> CATTAGCGTCAGACGATAAATTTAGCCGGAACTAAAACACTCTTGTATCATCGCCTTGTAGCG;> ATTAAAGATCGGCACGGAGATATCTTTGACCCCCACTAAAACCGCTTTT;> AAGGGCGACATTCAATAAGTTTACCAGAATGAAATTTTACAG;> TTTTTTTTTTTGGTTTACCAGCGCCACAATAGAAAGCAGA;> TTTTTTTTTTTAGTCAGAAGCAACTCCAACAGGTTTTTTTTTTT;> AAGCGGAGGAGAAGGAACCCTAAATCACCATCAATATGATTTTTTTTTTT;> TTGCATCAAATCAGTAAATATTCATTGACCAGAGGGGGTAATAGTAAAA;> CAAACGTGACTCCTCGCTAATTGAACAAAGTCAGACTCCTCA;> TATTTTGTCACAATAAGACAAGGAACCAGAGCCACCACCGTTTTTTTTTT;> AATTCGAGCTTCAAAGCGAACTCCTTTTCTGTAGCTCAACATGTTTTAA;> TGATAGACGGTTTTTCGCCCTTTGACGTTGGAGTCCACGTTCTTTAATAGTGGACTCTTGTTCCAAACTGGAACAACACTCAACCCTATCTCGGGCTATTCTTTTGATTTATAAGGGATTTTGCCGATTTCGGAACCACCATCAAACAGGATTTTCGCCTGCTGGGGCAAACCAGCGTGGACCGCTTGCTGCAACTCTCTCAGGGCCAG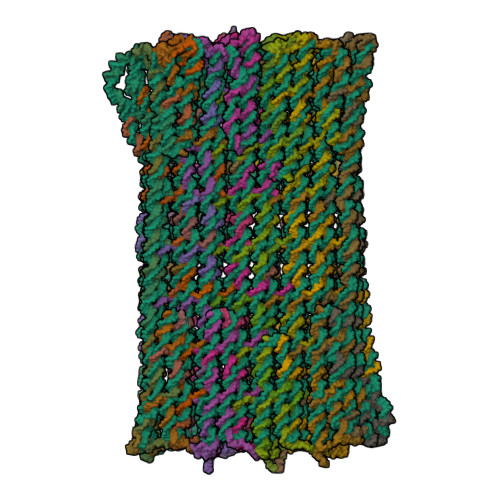GCGGTGAAGGGCAATCAGCTGTTGCCCGTCTCACTGGTGAAAAGAAAAACCACCCTGGCGCCCAATACGCAAACCGCCTCTCCCCGCGCGTTGGCCGATTCATTAATGCAGCTGGCACGACAGGTTTCCCGACTGGAAAGCGGGCAGTGAGCGCAACGCAATTAATGTGAGTTAGCTCACTCATTAGGCACCCCAGGCTTTACACTTTATGCTTCCGGCTCGTATGTTGTGTGGAATTGTGAGCGGATAACAATTTCACACAGGAAACAGCTATGACCATGATTACGAATTCGAGCTCGGTACCCGGGGATCCTCAACTGTGAGGAGGCTCACGGACGCGAAGAACAGGCACGCGTGCTGGCAGAAACCCCCGGTATGACCGTGAAAACGGCCCGCCGCATTCTGGCCGCAGCACCACAGAGTGCACAGGCGCGCAGTGACACTGCGCTGGATCGTCTGATGCAGGGGGCACCGGCACCGCTGGCTGCAGGTAACCCGGCATCTGATGCCGTTAACGATTTGCTGAACACACCAGTGTAAGGGATGTTTATGACGAGCAAAGAAACCTTTACCCATTACCAGCCGCAGGGCAACAGTGACCCGGCTCATACCGCAACCGCGCCCGGCGGATTGAGTGCGAAAGCGCCTGCAATGACCCCGCTGATGCTGGACACCTCCAGCCGTAAGCTGGTTGCGTGGGATGGCACCACCGACGGTGCTGCCGTTGGCATTCTTGCGGTTGCTGCTGACCAGACCAGCACCACGCTGACGTTCTACAAGTCCGGCACGTTCCGTTATGAGGATGTGCTCTGGCCGGAGGCTGCCAGCGACGAGACGAAAAAACGGACCGCGTTTGCCGGAACGGCAATCAGCATCGTTTAACTTTACCCTTCATCACTAAAGGCCGCCTGTGCGGCTTTTTTTACGGGATTTTTTTATGTCGATGTACACAACCGCCCAACTGCTGGCGGCAAATGAGCAGAAATTTAAGTTTGATCCGCTGTTTCTGCGTCTCTTTTTCCGTGAGAGCTATCCCTTCACCACGGAGAAAGTCTATCTCTCACAAATTCCGGGACTGGTAAACATGGCGCTGTACGTTTCGCCGATTGTTTCCGGTGAGGTTATCCGTTCCCGTGGCGGCTCCACCTCTGAAAGCTTGGCACTGGCCGTCGTTTTACAACGTCGTGACTGGGAAAACCCTGGCGTTACCCAACTTAATCGCCTTGCAGCACATCCCCCTTTCGCCAGCTGGCGTAATAGCGAAGAGGCCCGCACCGATCGCCCTTCCCAACAGTTGCGCAGCCTGAATGGCGAATGGCGCTTTGCCTGGTTTCCGGCACCAGAAGCGGTGCCGGAAAGCTGGCTGGAGTGCGATCTTCCTGAGGCCGATACTGTCGTCGTCCCCTCAAACTGGCAGATGCACGGTTACGATGCGCCCATCTACACCAACGTGACCTATCCCATTACGGTCAATCCGCCGTTTGTTCCCACGGAGAATCCGACGGGTTGTTACTCGCTCACATTTAATGTTGATGAAAGCTGGCTACAGGAAGGCCAGACGCGAATTATTTTTGATGGCGTTCCTATTGGTTAAAAAATGAGCTGATTTAACAAAAATTTAATGCGAATTTTAACAAAATATTAACGTTTACAATTTAAATATTTGCTTATACAATCTTCCTGTTTTTGGGGCTTTTCTGATTATCAACCGGGGTACATATGATTGACATGCTAGTTTTACGATTACCGTTCATCGATTCTCTTGTTTGCTCCAGACTCTCAGGCAATGACCTGATAGCCTTTGTAGATCTCTCAAAAATAGCTACCCTCTCCGGCATTAATTTATCAGCTAGAACGGTTGAATATCATATTGATGGTGATTTGACTGTCTCCGGCCTTTCTCACCCTTTTGAATCTTTACCTACACATTACTCAGGCATTGCATTTAAAATATATGAGGGTTCTAAAAATTTTTATCCTTGCGTTGAAATAAAGGCTTCTCCCGCAAAAGTATTACAGGGTCATAATGTTTTTGGTACAACCGATTTAGCTTTATGCTCTGAGGCTTTATTGCTTAATTTTGCTAATTCTTTGCCTTGCCTGTATGATTTATTGGATGTTAATGCTACTACTATTAGTAGAATTGATGCCACCTTTTCAGCTCGCGCCCCAAATGAAAATATAGCTAAACAGGTTATTGACCATTTGCGAAATGTATCTAATGGTCAAACTAAATCTACTCGTTCGCAGAATTGGGAATCAACTGTTATATGGAATGAAACTTCCAGACACCGTACTTTAGTTGCATATTTAAAACATGTTGAGCTACAGCATTATATTCAGCAATTAAGCTCTAAGCCATCCGCAAAAATGACCTCTTATCAAAAGGAGCAATTAAAGGTACTCTCTAATCCTGACCTGTTGGAGTTTGCTTCCGGTCTGGTTCGCTTTGAAGCTCGAATTAAAACGCGATATTTGAAGTCTTTCGGGCTTCCTCTTAATCTTTTTGATGCAATCCGCTTTGCTTCTGACTATAATAGTCAGGGTAAAGACCTGATTTTTGATTTATGGTCATTCTCGTTTTCTGAACTGTTTAAAGCATTTGAGGGGGATTCAATGAATATTTATGACGATTCCGCAGTATTGGACGCTATCCAGTCTAAACATTTTACTATTACCCCCTCTGGCAAAACTTCTTTTGCAAAAGCCTCTCGCTATTTTGGTTTTTATCGTCGTCTGGTAAACGAGGGTTATGATAGTGTTGCTCTTACTATGCCTCGTAATTCCTTTTGGCGTTATGTATCTGCATTAGTTGAATGTGGTATTCCTAAATCTCAACTGATGAATCTTTCTACCTGTAATAATGTTGTTCCGTTAGTTCGTTTTATTAACGTAGATTTTTCTTCCCAACGTCCTGACTGGTATAATGAGCCAGTTCTTAAAATCGCATAAGGTAATTCACAATGATTAAAGTTGAAATTAAACCATCTCAAGCCCAATTTACTACTCGTTCTGGTGTTTCTCGTCAGGGCAAGCCTTATTCACTGAATGAGCAGCTTTGTTACGTTGATTTGGGTAATGAATATCCGGTTCTTGTCAAGATTACTCTTGATGAAGGTCAGCCAGCCTATGCGCCTGGTCTGTACACCGTTCATCTGTCCTCTTTCAAAGTTGGTCAGTTCGGTTCCCTTATGATTGACCGTCTGCGCCTCGTTCCGGCTAAGTAACATGGAGCAGGTCGCGGATTTCGACACAATTTATCAGGCGATGATACAAATCTCCGTTGTACTTTGTTTCGCGCTTGGTATAATCGCTGGGGGTCAAAGATGAGTGTTTTAGTGTATTCTTTTGCCTCTTTCGTTTTAGGTTGGTGCCTTCGTAGTGGCATTACGTATTTTACCCGTTTAATGGAAACTTCCTCATGAAAAAGTCTTTAGTCCTCAAAGCCTCTGTAGCCGTTGCTACCCTCGTTCCGATGCTGTCTTTCGCTGCTGAGGGTGACGATCCCGCAAAAGCGGCCTTTAACTCCCTGCAAGCCTCAGCGACCGAATATATCGGTTATGCGTGGGCGATGGTTGTTGTCATTGTCGGCGCAACTATCGGTATCAAGCTGTTTAAGAAATTCACCTCGAAAGCAAGCTGATAAACCGATACAATTAAAGGCTCCTTTTGGAGCCTTTTTTTTGGAGATTTTCAACGTGAAAAAATTATTATTCGCAATTCCTTTAGTTGTTCCTTTCTATTCTCACTCCGCTGAAACTGTTGAAAGTTGTTTAGCAAAATCCCATACAGAAAATTCATTTACTAACGTCTGGAAAGACGACAAAACTTTAGATCGTTACGCTAACTATGAGGGCTGTCTGTGGAATGCTACAGGCGTTGTAGTTTGTACTGGTGACGAAACTCAGTGTTACGGTACATGGGTTCCTATTGGGCTTGCTATCCCTGAAAATGAGGGTGGTGGCTCTGAGGGTGGCGGTTCTGAGGGTGGCGGTTCTGAGGGTGGCGGTACTAAACCTCCTGAGTACGGTGATACACCTATTCCGGGCTATACTTATATCAACCCTCTCGACGGCACTTATCCGCCTGGTACTGAGCAAAACCCCGCTAATCCTAATCCTTCTCTTGAGGAGTCTCAGCCTCTTAATACTTTCATGTTTCAGAATAATAGGTTCCGAAATAGGCAGGGGGCATTAACTGTTTATACGGGCACTGTTACTCAAGGCACTGACCCCGTTAAAACTTATTACCAGTACACTCCTGTATCATCAAAAGCCATGTATGACGCTTACTGGAACGGTAAATTCAGAGACTGCGCTTTCCATTCTGGCTTTAATGAGGATTTATTTGTTTGTGAATATCAAGGCCAATCGTCTGACCTGCCTCAACCTCCTGTCAATGCTGGCGGCGGCTCTGGTGGTGGTTCTGGTGGCGGCTCTGAGGGTGGTGGCTCTGAGGGTGGCGGTTCTGAGGGTGGCGGCTCTGAGGGAGGCGGTTCCGGTGGTGGCTCTGGTTCCGGTGATTTTGATTATGAAAAGATGGCAAACGCTAATAAGGGGGCTATGACCGAAAATGCCGATGAAAACGCGCTACAGTCTGACGCTAAAGGCAAACTTGATTCTGTCGCTACTGATTACGGTGCTGCTATCGATGGTTTCATTGGTGACGTTTCCGGCCTTGCTAATGGTAATGGTGCTACTGGTGATTTTGCTGGCTCTAATTCCCAAATGGCTCAAGTCGGTGACGGTGATAATTCACCTTTAATGAATAATTTCCGTCAATATTTACCTTCCCTCCCTCAATCGGTTGAATGTCGCCCTTTTGTCTTTGGCGCTGGTAAACCATATGAATTTTCTATTGATTGTGACAAAATAAACTTATTCCGTGGTGTCTTTGCGTTTCTTTTATATGTTGCCACCTTTATGTATGTATTTTCTACGTTTGCTAACATACTGCGTAATAAGGAGTCTTAATCATGCCAGTTCTTTTGGGTATTCCGTTATTATTGCGTTTCCTCGGTTTCCTTCTGGTAACTTTGTTCGGCTATCTGCTTACTTTTCTTAAAAAGGGCTTCGGTAAGATAGCTATTGCTATTTCATTGTTTCTTGCTCTTATTATTGGGCTTAACTCAATTCTTGTGGGTTATCTCTCTGATATTAGCGCTCAATTACCCTCTGACTTTGTTCAGGGTGTTCAGTTAATTCTCCCGTCTAATGCGCTTCCCTGTTTTTATGTTATTCTCTCTGTAAAGGCTGCTATTTTCATTTTTGACGTTAAACAAAAAATCGTTTCTTATTTGGATTGGGATAAATAATATGGCTGTTTATTTTGTAACTGGCAAATTAGGCTCTGGAAAGACGCTCGTTAGCGTTGGTAAGATTCAGGATAAAATTGTAGCTGGGTGCAAAATAGCAACTAATCTTGATTTAAGGCTTCAAAACCTCCCGCAAGTCGGGAGGTTCGCTAAAACGCCTCGCGTTCTTAGAATACCGGATAAGCCTTCTATATCTGATTTGCTTGCTATTGGGCGCGGTAATGATTCCTACGATGAAAATAAAAACGGCTTGCTTGTTCTCGATGAGTGCGGTACTTGGTTTAATACCCGTTCTTGGAATGATAAGGAAAGACAGCCGATTATTGATTGGTTTCTACATGCTCGTAAATTAGGATGGGATATTATTTTTCTTGTTCAGGACTTATCTATTGTTGATAAACAGGCGCGTTCTGCATTAGCTGAACATGTTGTTTATTGTCGTCGTCTGGACAGAATTACTTTACCTTTTGTCGGTACTTTATATTCTCTTATTACTGGCTCGAAAATGCCTCTGCCTAAATTACATGTTGGCGTTGTTAAATATGGCGATTCTCAATTAAGCCCTACTGTTGAGCGTTGGCTTTATACTGGTAAGAATTTGTATAACGCATATGATACTAAACAGGCTTTTTCTAGTAATTATGATTCCGGTGTTTATTCTTATTTAACGCCTTATTTATCACACGGTCGGTATTTCAAACCATTAAATTTAGGTCAGAAGATGAAATTAACTAAAATATATTTGAAAAAGTTTTCTCGCGTTCTTTGTCTTGCGATTGGATTTGCATCAGCATTTACATATAGTTATATAACCCAACCTAAGCCGGAGGTTAAAAAGGTAGTCTCTCAGACCTATGATTTTGATAAATTCACTATTGACTCTTCTCAGCGTCTTAATCTAAGCTATCGCTATGTTTTCAAGGATTCTAAGGGAAAATTAATTAATAGCGACGATTTACAGAAGCAAGGTTATTCACTCACATATATTGATTTATGTACTGTTTCCATTAAAAAAGGTAATTCAAATGAAATTGTTAAATGTAATTAATTTTGTTTTCTTGATGTTTGTTTCATCATCTTCTTTTGCTCAGGTAATTGAAATGAATAATTCGCCTCTGCGCGATTTTGTAACTTGGTATTCAAAGCAATCAGGCGAATCCGTTATTGTTTCTCCCGATGTAAAAGGTACTGTTACTGTATATTCATCTGACGTTAAACCTGAAAATCTACGCAATTTCTTTATTTCTGTTTTACGTGCAAATAATTTTGATATGGTAGGTTCTAACCCTTCCATTATTCAGAAGTATAATCCAAACAATCAGGATTATATTGATGAATTGCCATCATCTGATAATCAGGAATATGATGATAATTCCGCTCCTTCTGGTGGTTTCTTTGTTCCGCAAAATGATAATGTTACTCAAACTTTTAAAATTAATAACGTTCGGGCAAAGGATTTAATACGAGTTGTCGAATTGTTTGTAAAGTCTAATACTTCTAAATCCTCAAATGTATTATCTATTGACGGCTCTAATCTATTAGTTGTTAGTGCTCCTAAAGATATTTTAGATAACCTTCCTCAATTCCTTTCAACTGTTGATTTGCCAACTGACCAGATATTGATTGAGGGTTTGATATTTGAGGTTCAGCAAGGTGATGCTTTAGATTTTTCATTTGCTGCTGGCTCTCAGCGTGGCACTGTTGCAGGCGGTGTTAATACTGACCGCCTCACCTCTGTTTTATCTTCTGCTGGTGGTTCGTTCGGTATTTTTAATGGCGATGTTTTAGGGCTATCAGTTCGCGCATTAAAGACTAATAGCCATTCAAAAATATTGTCTGTGCCACGTATTCTTACGCTTTCAGGTCAGAAGGGTTCTATCTCTGTTGGCCAGAATGTCCCTTTTATTACTGGTCGTGTGACTGGTGAATCTGCCAATGTAAATAATCCATTTCAGACGATTGAGCGTCAAAATGTAGGTATTTCCATGAGCGTTTTTCCTGTTGCAATGGCTGGCGGTAATATTGTTCTGGATATTACCAGCAAGGCCGATAGTTTGAGTTCTTCTACTCAGGCAAGTGATGTTATTACTAATCAAAGAAGTATTGCTACAACGGTTAATTTGCGTGATGGACAGACTCTTTTACTCGGTGGCCTCACTGATTATAAAAACACTTCTCAGGATTCTGGCGTACCGTTCCTGTCTAAAATCCCTTTAATCGGCCTCCTGTTTAGCTCCCGCTCTGATTCTAACGAGGAAAGCACGTTATACGTGCTCGTCAAAGCAACCATAGTACGCGCCCTGTAGCGGCGCATTAAGCGCGGCGGGTGTGGTGGTTACGCGCAGCGTGACCGCTACACTTGCCAGCGCCCTAGCGCCCGCTCCTTTCGCTTTCTTCCCTTCCTTTCTCGCCACGTTCGCCGGCTTTCCCCGTCAAGCTCTAAATCGGGGGCTCCCTTTAGGGTTCCGATTTAGTGCTTTACGGCACCTCGACCCCAAAAAACTTGATTTGGGTGATGGTTCACGTAGTGGGCCATCGCCC;> TTTTTTTTTTACTAAAGACTTTTTCATACAGAGGGAGCCT;> TTTTTTTTTTACAGACCAGGCGAGCTGCTCATTCTTTTTTTTTT;> CATAGGCTGGCTGATTTGAAAGAGGACAGATGAACGGTGTTTTTTTTTTT;> CCTTCATTTACCCAAACACCAAATTTCACCAGTCAGGACGTTGGGAA;> GGCTTGCGACAACATAAACAAGTCTTTCCAGACGTTAGTAAAGTATGGG;> CTCAGCAGAATTTCAACAACTCAGACAGCCCTCATAGTTAGCTGAGAAT;> AGGGTAGCAACGGCTGAGGAAGTTTCCATTAAACGCGGAACGTTATCAG;> GTTGCGCCGACAATAGGGAGTCAGAGCCCGTTTTCGTGAATTATCACAA;> ACCGATAAGCGGAGGTAACGATCTAAAGTTTTGTCCTTTCAA;> TTAAACAGCTTGATGCGGGATAGCCGCCTCATAGCGACGGAATTAGAGCCAGCA;> TTTTTTTTTTGCTCCAAAAGCTTTGAGGTTTTTTTTTT;> TTTTTTTTTTAGTGAATAAGGCGAATTACCTTATTTTTTTTTTT;> TAATAATTACAACGTTTCAGGGATAGCATACCGCC;> AATCTCCAGTTTCGTAGGAACCCATGTACCTTTTTTTTTT;> ACTTTAATCATTGTTTGCCCTAATTACGCGTTTACGAAGCAA;> TGAATGGGCTTGAGATGGTTTGAACGAGCAGATAC;> CCTGTAGCATTCCAAAAGGAAGGGTCAGAAAGCGCCGAGGAAAAAGACA;> TCACCAGTACAAACTTTTTCATACTGGTCCGTTCCACAAAGT;> TTTTTTTTTTGTAACACTGAAAAAAAAGTTTTTTTTTT;> AGCGCGAAACAAAGTACAATTTTCGGACCAGAAAAATAAATATAAAC;> ACCTGCTCCCAATCATACCGATATATTCGGCAGGAGG;> GAAAAATCTACGTTCAACTTATAATGGATAAGAAATAGTATAAAGCTAAATCGG;> TTTTTTTTTTCCGTACTCAGGAGGTTTAGAGCCCAA;> TTTTTTTTTTGCGATTTTAAGAACTGGCTTAACGGA;> ACCCTCAGAGCCACCACACCCTCTGCCGTCAACATAAAAGAGCA;> TTTTTTTTTTTAGAAAGATGTAAGAGCATTTTTTTTTT;> TTGAGATTTAGGAACAAAAGGGACGAGAAATCAACGTAACAA;> GGGTTTTGCTCAGTATTAGACAATTGAGTTTTATTCAAGAAATCATTTG;> GAGAGGGTTTAACGTTGCGAACTTGCTTTCGAGGTGCGAAAG;> AAGTATAAGCAGCCAGCAATATATTAAAACCAATCAAACAAA;> GCCCGGAAGGAGTGCGTTGAATTAATTGTATCGGT;> AGGCATATCATCAGACAACATTATTACAGGTTTTTTTTTT;> TCTGAAACATGATGTAGTAAAGAACCGGATATTCACAAGAGT;> CTATTATGGCAGGTCAATATCGCGTTTTTTTGCGGATGGCGT;> TCGGAACATTTTGCACCATCGCCCACGCATAACAATTTTTCT;> GCCCCCTTGATATTTGATTAAAGAAAATCAGACGAAGTATCA;> GTGCCCGTCCTCATGAATACCGGCAACAAAAAGGTATTCTTA;> TTTTTTTTTTTTTTGATGATACATAGGTGTATCATTTTTTTTTT;> TTTTTTTTTTACACTATCAACTGGATAGTTTTTTTTTT;> CAGACGACGATAAAATAACGCTACCACATTAATAAAACGAACCATTATA;> AACCAAAATAGCGACAAAAGAAATCTTGAAGGGAACCGAACTGACCAAC;> TAAAGCCCCCTCAGCGTCACCACGAAGGCACCAACGCGATTATACCA;> GAATTTAAATAAGTTTGATATACCCTCAGAACCGCCCCTCAT;> AGTTTTGATCCCCCTGACCATAAATCAAAAAAAGATTAAGAG;> GCATTGATCGCTGAGAGGCGCAGACGGTATGTTACTGTGTCGAAATCCGCG;> GCCGCCATTGGCCTGCCTATTAGAGAAGGATTAGGAACACCCATCAGAG;> GCCACCAAGAATGGTGCCTTGGGATAAGAGAACCGCC;> CCTCAGATTGCCATGAGGGAGGGAAGGTGAAACGCACGCAAT;> TTTTTTTTTTGAACCGCCTCCCGTCATACATGGCTTTTTTTTTT;> TTTTTTTTTTCGTCCAATACTGCGGATGTTTAGTAACCCT;> ATCGTCAGTCTTTACCCTGACTATTATTTTTTTTTT;> GATTAAGAATCATATCGCCATATTTAACAACGCTTTTTTTTTT;> AGGTCATTGCCTGAAGAGGGTAACCAGGCAGCTGGTGGGTAACGCCAGG;> TTTTTTTTTTTACCTGAGCGAAGAGTCATTTTTTTTTT;> TTTTTTTTTTTAATCGTAAAACATTTTGTTAAAATTTTTTTTTT;> TATGTACATTTAAACTCATTTTTTAACCGGCCTTC;> ACATCGGTTTTTTAAGATAAGTTCTGTCACATACA;> CTGATTGTTTGCACGTAAAACTCCCGACAAGCCGTTTAAGCCAATAACG;> TTACAAAGAACCTAAGATGATGGCAATTCCAGAAGTTAAAAGTTTGAGT;> ATCGCGCCAGTTGGCACCTTGAGAAAGCAACAGGAGGCCGAT;> AATTATTTTCTGAAATAATCCTGATTGTTTTTTTTT;> ACTGGCACACAAACCCACCACTAAAGGCGAAAGAGGCAAAAGAATACAC;> CAAAAGACCACAAGGGGAGAATTAACTGATTAGCGAGTTAATCAGTTTC;> AGGAAACAGTCTCTCCGCCACACAGCATGGTAAAATACGTAATGCCACT;> TTTTTTTTTTAAGAAAAGTAAATTCATATTTTTTTTTT;> TTTTTTTTTTCAGGATTAGAGAATATGCAACTAATTTTTTTTTT;> GTACCTTCAATAAAAAGCAATCAAGAGATAGCTGATAAATTA;> CAATAATAAACAGGGAAGCGCACCAGGCAGTAACAAGAAAGG;> TACCGAATCAAAAAATAAGAAACGATTTTTTTTTTTTTTT;> GGTTAGAGCTTAATTGCTGAAAAAAGTATTAAGAGGCTGAGA;> TTTTTTTTTTTGTTTAACGGCCCTTTTTTTTTTTTTTT;> ATTCTGCGAACGCGCGAGCAGCAAATCCCGGTT;> TTTTTTTTTTTACAATTTTATCCTGAATCAATCCAATGAAAAT;> TTTTTTTTTTAGTACGGTGTCTGGAAGTTGACCATTTAGCTAT;> TGCCAGTTACAAAATATTTCCAGAGGTTTTAAAATTACTTTGAAAAAGGAA;> ATATTATTTATCCCTTACCAAAGATTAGAGGGTTA;> AAATCACCAGTAGCACCATTATACAAAAAGTAATCCTGAA;> GCAGCACCGTCAGAAAGAAAGACTTCAAGTATGTTCA;> TTTTTTTTTTTGGTCAATAGGCAAGGCATTTTTTTTTT;> TTTGGGGAGTAGATTTAGTTTTCATTCCATATAACAGTTGATTCCCA;> GTGGCATATAGAAGTGAAAACAGGAAGAACGCCATCA;> TCATACAACCTGTTAGATACATTTCGCAAATTTTTTTTTT;> GCAAATCATGCAGAATACAAAGGCTATCAGAAAAGCCCCAAA;> CATTACCCAACAATATGGAAACCTTGCTAAAAATA;> TTCATCGCGTTTTAGCGAACCAGAAATAAATAACGCTAAAAT;> CATCGAGCTAATTTAATTAATGAATCCTTGAAAAC;> CCAAGTATAAATCACGCTAACGAGCGTCAACAGCCAGAGAAT;> GAACGGGGCTATCTTAGCCGAAGTAAGCTCAGAGCCGCCACCCTCAGAA;> TTTTTTTTTTTTATCATTCCAATTTGCACCCAGCTTTTTTTTTT;> TTTTTTTTTTAAGAATTAGTTCAACGCATTTTTTTTTT;> AATAATATACCGACTATAAAAAAATATTCCCCTTATTAGCGT;> ACGAGCACAGTAATCCACGGAACCGATTCTTTTCATAATCAAAATCACC;> TGACCCTGCAATGCTGAGAAAGGCCGGAATGCCGGGAGTCTG;> AACATTAGAAGCCCACGAGAATCAAATGCTTTAAATTTTTTGGAGGCGA;> AAACAACATGTTAGTCAAGTTTGCCTGTTAATCAGAATGAAACCATCGATA;> CGACAATTGTTTATGCGCCCACGGTATTCTAAGAA;> TATAAAGTCCCATCAACAAGCTTGCGGGAGCCTAATT;> AAGAGAAACGCTCAAACCTCCGGCTTAGTCCCTTATACATTT;> TTTTTTTTTTCAACATGTAATTGGCTGTCTTTCCTTTTTTTTTT;> TTTTTTTTTTAGGATAAAAATTTTTACCTTTATCAAAATT;> GGTACTAGAAAAAGCGTCACCTAGCGACAGCGTCACCGACTTAGCAAGGCCGGAAACCTGTTT;> TTGAGAAGGTCTGAGAGACTAATAGCGACATCAAG;> GACAGTCCATATATTTTAAATGTAATACCAGAGCAGTAGCAT;> ATAAGAAGACCGTGTAGTTAATTTCATCATGGATTCCGAACG;> GCGTTAATATGCGTTACCATTGAGCCATTTGGGAAATTATTCTAAAGGT;> TATATAACTATAAGATCGTCGAATTACCGAGAAAC;> CCTTTTTACAGTAGGGCTTAATTCGAGCTGTAGAA;> TTTTTTTTTTATAGTGAATTTATCAAACGCTGAAAAAGAA;> TTTTTTTTTTATTCAACCGTTCATCGATGAACGGTTTTTTTTTT;> AGCTATTAAAAGGGCTGAGTAATGTGTAGCCCAAATTGTATAAGATCAA;> TTTGAGAGATCTATAGCAGAAGCCAATCGTCTGAATTCTGACCTAAA;> CTATTAATAGCCCTAGTCACACTGTCCATTGCCTGAGTAG;> TAGCTTACAATATTGATAGAAAGAAGTGTTTTTATGGAGCTAGAAAGGA;> GACGGGGATCGGCAAATCCTGTTTGATGGTTTTTTTTTTT;> ATCAAACGGTGAAGAACGTCAAGAATGCCAACGGCGCGCTTT;> ACAGCGGGGGAACACGTAACCTCAATCAGAGCAAAAAAGCCTTTTTGCG;> AAGAACGTGGACTCTTGAGGATTAGAGCTATACAGTAAATCAACGCGCC;> GGGTTGAGTGTTGTCTCGTATAGGTTATGATTCGCAACAATT;> AAATCCCTTATAAACCGATTTACATACGAGCTGTTTCCTGTG;> TTTTTTTTTTGGTTCCGAAAAAGCCGGCTTTTTTTTTT;> AAATCCCGTAAATCCGTTTTTTCGTCCTCATAATATCAGG;> TTTTTTTTTTCTTTTCACCAGTGAGACGGAGGCGAA;> TTTTTTTTTTTCATTTGCCGCCAGCAGTTCGGCCTTTTGCCGTTCCGGCA;> CGTTAATTAGCATGGTGCATCCTCAGGACCGGAAT;> TTGTAAAATTTTCATAACATCTAATTGCCAGACCG;> GGTTTAACGTCAGAGCTTATCATAGCAAAATTGAGTATTACGCAGACGA;> ATTTTCAACCTTTTTAACAACTATTAACCCACACCACTATGG;> AAGAAATTGCGTAGCGCGAGGTAGGAATAGATAAC;> TTTTTTTTTTGGATTATACCATTTCAATTTTTTTTTTT;> AAAATAATTCGCGTCTAATAGGATTGTATATGAAAAGTTCTACTGGTCATT;> TTTTTTTTTTTTGCGGAACAAAGAAACCACATCAATTAATGGATTGCTAT;> TTTTTTTTTTTTCGCATTAAATTTTTGTTCATCAACTCTCCGT;> TTCCTGATTATCCCATATCGAAGCCTCCGCACTAGAAACA;> AGACAAAGATAATAAAAATGCGCCCAGCAGTTGAGGA;> TTTAATGGTTTGAAATACCTAAACACTGAATAACAGTACATAACAGT;> TTTTTTTTTTTAACAACCCTTGAGGGGATTTTTTTTTT;> GATTGACCGAGAGACGCAGAATGTGTACATCGACATAAAA;> CGTAATGGGATAATAATACATCAACGTCCCCACTAGGCCAGA;> TAAATCCTTTGCCCCGAGATATCGGAACAGTGTAA;> TGCCAGTGTCGGATATTAAATGTGAGCGAGTTTTTTTTTT;> GTAGATGCCAGCTTACAGCGCCGCCACGCGGGGTC;> CGTCAATAAACAGACGGAAACAATCGGCGCGATGGAAAGGGCGAAAAAC;> ATCTGGTAGAGGCGGATGATGAATAATCTAGGCAGAGGCATT;> TTTTTTTTTTCCCTCAATCAATAACATTATCATTTTTTTTTTTT;> TTTTTTTTTTCGACGACAGCAACTGTTGTTTTTTTTTT;> ACTCCAGGGCGCATAACGGCGCTGTAGCCAGCTTTAAATCAG;> GGTGAGGAACCACCATGTGAGCGGAATCATAATTAAAGATTC;> CGGTCAGTAATAGATTTAGAAGTATTAGACTATTACAAATCATAATTGC;> TGCCACGCGGTCACACGTATATTTCACGGTTAACGGCATCAGATGCCGG;> CTGAGAGGAACTGATTAATTTGTTGGGTCCAGTATAAAGCCA;> CAAATGACTAGGGCTTAGAATGGCCAGAGTTACCTGCAGCCAGCGGTGC;> AAAACATGCAACAGATCTTTAAAACAATTCGACAATCCAGTT;> TTTGAATAAAGCATCAAATCAATTAATTGAGCGGAATTATCATCATA;> TTTTTTTTTTTAAGAATACGTGTCAAATATCAAATTTTTTTTTT;> TTTTTTTTTTGGAAGGGCGATCGGTGGGCTGCGTATCGGC;> CGGGCCTCAGTCACGACGTTGTAAAATTTTTTTTTT;> ATTTACACGTTGTAGCAATTAGGCGCGTCGCCGCGCATCACC;> TTGGCAGTATATTTTGATAAATATGTAAATGCTGAAAAACTTTTTCAAAATTCACC;> GAGGCCACCGAGTATTCCTCGGCTGGCACACTAAA;> AATCCTGCCCTTCTGACCTGAAAGCGTTTTTTTTTT;> TTTTTTTTTTAGGAACGGTACGCCAGTAAAGGGGAGAAAG;> TTTTTTTTTTCGACGGCCAGTGTTGTGAGAGATATTTTTTTTTT;> CCAAGCTCGCACTCGTCACTGTTGCCCTGCGGCTGATTGCAG;> TTCAGAGGTTTTCCCTTCGCTATTACGCCAAAGCG;> GTGGAGCCATGTTTTCTCACGGAAAATCCGGAACGTCGGTGGTGCCATC;> GCTACAGCATTTTGACGCTTGCGCTCATCCGCCAGCCATTGCAA;> GACGAGCGCTGCGCTGGGGTCTGGAACAAGAGTCCACTTTACGGAGCAC;> ACGTGCTAAAGAGTCGACCAGACGCGAGTGCAAATCCAATCGCA;> GAAACGTTCCGGCACCGCTTAAGGGTCACGTTGGTGATAATC;> TTTTTTTTTTGAACGTGGCATTTTAGACTTTTTTTTTT;> TTTTTTTTTTGACTTTCTCCGTTTAAATTTCTGCTTTTTTTTTT;> AGTTTTTGTAACCAACCGCCTCGCCATTTCTGTAA;> GAGGTGCAATGAGTAGGATCCCCGGGTAGGGCCGT;> CCTAAAGGCGGGCGAAAATCTGGCTATTAGTCTTTAGGGACA;> GGAGCCCTCAAAAGTGGTTTGCCCCAGCGCAACAGGCGTATTGGGCGCC;> GAGTTGCAGCAAGCGGCCGCCTGACGCGCGGGGAGAGAGCATAA;> TCCACGCAATAGCCGAACGTTACAGTTGTACCAAGAAAACAA;> GTAATATCCAGAACTCCCTTAAGCACGCGTGCCCG;> AAGAACTCAAACTATCGGCGCAAATCGTCATACACAGTTGGAGCTAA;> CAGGAAAAACAAGGCGATAACCTCACCGCCGCTGGAG;> TTTTTTTTTTAGTTAAACGGCTGGTCTGTTTTTTTTTT;> TCGTCGCTGGCAGCCTGCCCGCTTTCCAGTCGGGAAACCTGTCTCACAT;> CGTGCCAGCTGCATTAATGAAGGTGCCTCGTAAAGAGTGTAG;> GCGTGGTATGCTGATAGTGATGAAGGGTAATTTTTTTTTT;> CTTGTAGGGATAGCACCAGTCAGATCGCCCATTCGCCATTCA;> CCACACAAGAGCTTGAAGGGACTGAACCGCACAGA;> TTTTTTTTTTCCGCTCACAATTAGGGTGGTTTTTTTTTTTTTTT;> TTTTTTTTTTGTCAGCAGCCGGGCGCGGTTTTTTTTTT;> AGCACCGTGCCGGAAACGCGGAAAAGCCGCACAGGGGGCGGT;> ACCAGCTTATGTTCTTCGCGTGTTGCGCTCACTCCCGTGAACCTTAATG;> CCGTGAGCCTCCTCCGGGGGTTTGCTTTAATTAAC;> CGAATTCGTAATCAGTGCTGCCAGAGCGAATCAGTTTCTGGCCAACAGA;> GCATCAGGGAACGGATTAAGTCGAAAGGGGGATGTGATCTGGTGCCGGA;> TTCTGCCCACTGGTGTGTTCACTTGCTGAGTAATAACATCACTCACGCA;> ATGCGGCCCGAGCTAGCCTGGTCGGCCAGCCCTGAGA;> CTCTGTGTGGTCATAGCCGGAGCGGTTTCTGATTGCCCTTCA;> TGCGCGCCTGTGCACGGTGCCCCCTGCATCAGACGATCCATTTTTTTTTT;> TTTTTTTTTTGCGCAGTGTCACTGAAATTGTTATTTTTTTTTTT;> TTTTTTTTTTTTGCGGTATGAGCCGGAATCCGCAACCGCA;> GTAATGGGTAAAGGTTTCTTTGTGTCCACCACGCAGCACATC;> GCTCGTCATAAACAAATATTAGGAAATACCACTTCTTTGATT> MINNPKVDSVAEKPKAVTSKQSEQAASPEPTPAPPVSRNQYPITFNLTSTAPFHLHDRHRYLQEQDLYKCASRDSLSSLQQLAHTPNGSTRKKYIVEDQSPYSSENPVIVTSSYNHTVCTNYLRPRMQFTGYQIS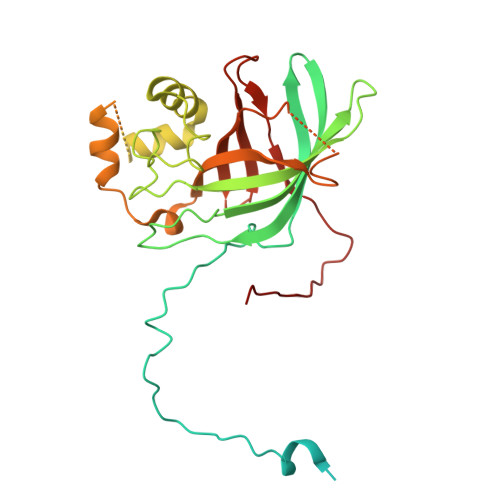GYKRYQVTVNLKTVDLPKKDCTSLSPHLSGFLSIRGLTNQHPEISTYFEAYAVNHKELGFLSSSWKDEPVLNEFKATDQTDLEHWINFPSFRQLFLMSQKNGLNSTDDNGTTNAAKKLPPQQLPTTPSADAGNISRIFSQEKQFDNYLNERFIFMKWKEKFLVPDALLMEGVDGASYDGFYYIVHDQVTGNIQGFYYHQDAEKFQQLELVPSLKNKVESSDCSFEFA>MHHHHHHENLYFQSMASGTTTTAVKIGIIGGTGLDDPEILEGRTEKYVDTPFGKPSDALILGKIKN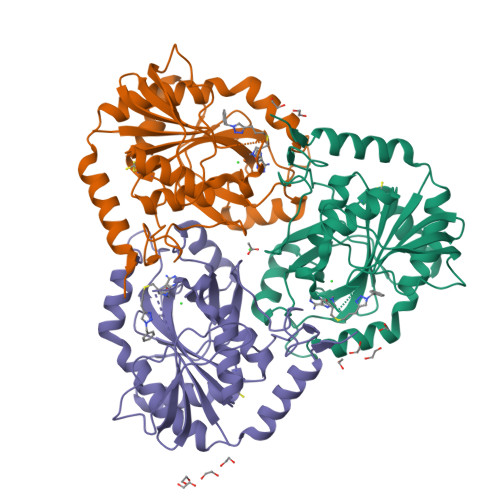VDCVLLARHGRQHTIMPSKVNYQANIWALKEEGCTHVIVTTACGSLREEIQPGDIVIIDQFIDRTTMRPQSFYDGSHSCARGVCHIPMAEPFCPKTREVLIETAKKLGLRCHSKGTMVTIEGPRFSSRAESFMFRTWGADVINMTTVPEVVLAKEAGICYASIAMATDYDCWKEHEEAVSVDRVLKTLKENANKAKSLLLTTIPQIGSTEWSETLHNLKNMAQFSVLLPRH[3x]>GAMERVLKVFHYFENSSEPTTWASIIRHGDATDVRGIIQKIVDCHKVKNVACYGLRLSHLQSEEVHWLHLDMGVSNVREKFELAHPPEEWKYELRIRYLPKGFLNQFTEDKPTLNFFYQQVKNDYMLEIADQVDQEIALKLGCLEIRRSYGEMRGNALEKKSNYEVLEKDVGLRRFFPKSLLDSVKAKTLRKLIQQTFRQFANLNREESILKFFEILSPVYRFDKECFKCALGSSWIISVELAIGPEEGISYLTDKGANPTHLADFNQVQTIQYSNSEDKDRKGMLQLKIAGAPEPLTVTAPSLTIAENMADLIDGYCRLVNGATQSFIIRPQKEGERALPSIPKLANNEKQGVRSHTVSVSETDDYAEIIDEEDTYTMPSTRDYEIQRERIELGRCIGEGQFGDVHQGIYMSPENPAMAVAIKTCKNCTSDSVREKFLQEALTMRQFDHPHIVKLIGVITENPVWIIMELCTLGELRSFLQVRKFSLDLASLILYAYQLSTALA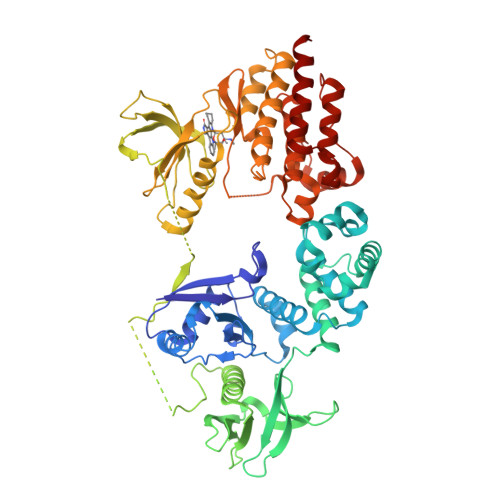YLESKRFVHRDIAARNVLVSATDCVKLGDFGLSRYMEDSTYYKASKGKLPIKWMAPESINFRRFTSASDVWMFGVCMWEILMHGVKPFQGVKNNDVIGRIENGERLPMPPNCPPTLYSLMTKCWAYDPSRRPRFTELKAQLSTILEEEKLQ[2x]> KETCAAKFERQHMDSS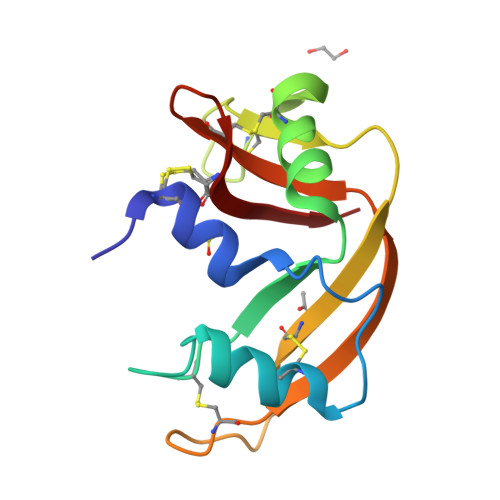TSAASSSNYCNQMMKSRNLTKDRCKPVNTFVHESLADVQAVCSQKNVACKNGQTNCYQSYSTMSITECRETGSSKYPNCAYKTTQANKHIIVACEGNPYVPCHFDASV>AVDIRDVKISFPGTQNPKFPHLRFMQTLPAVRQLTVCQRIKPFHRNTGYIFSCATSNQDNQFITSMYVKSDGTLNLGLQVNASSNKYISCPIEIELGQWYHVCHVWSGVDGRMAVYANGSPCGTMENVGKGHQISAGGTVVIGQEQDKIGGGFEEQESWSGELSDLQVWDEALTTHQVST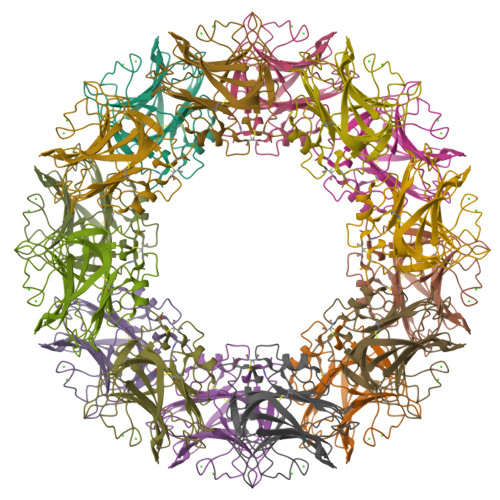VASCNGIRPRGNVISWMEDSFVADDGVIVGISHMCSL[2x]> DPMAAGFKTVEPLEYYRRFLKENCRPDGRELGEFRTTTVNIGSISTADGSALVK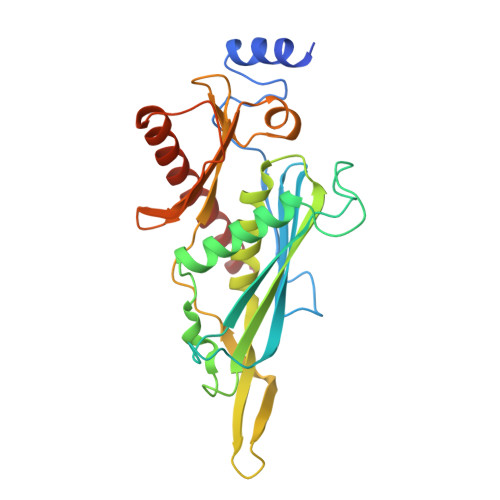LGNTTVICGVKAEFAAPSTDAPDKGYVVPNVDLPPLCSSRFRSGPPGEEAQVASQFIADVIENSQIIQKEDLCISPGKLVWVLYCDLICLDYDGNILDACTFALLAALKNVQLPEVTINEETALAEVNLKKKSYLNIRTHPVATSFAVFDDTLLIVDPTGEEEHLATGTLTIVMDEEGKLCCLHKPGGSGLTGAKLQDCMSRAVTRHKEVKKLMDEVIKSMKPK methyl 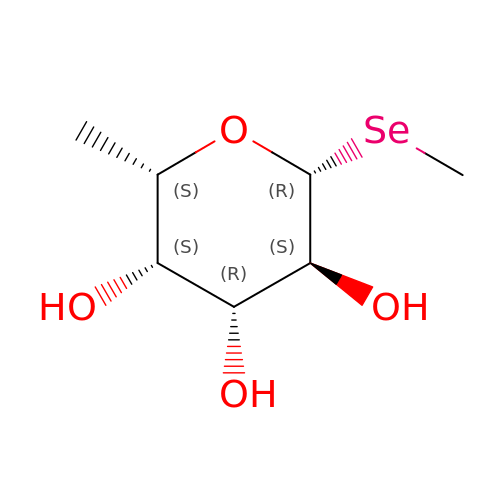1-seleno-beta-L-fucopyranoside | C7 H14 O4 Se | VHTNTJQSKJZERS-CXNFULCWSA-N> MEAYLNKIDKIEPSDQKIKEEYNKFKYDITKQAIESLRERIPKRIIFFNNLVNVNSEPGSILNVNDLDGVSYKYKINKIEENVRKKHKGNNSSDFDEREKKKDSLDGHVKHFSNNEDSKLIIDDKVLYTHYVPSHKQIYLELEKIK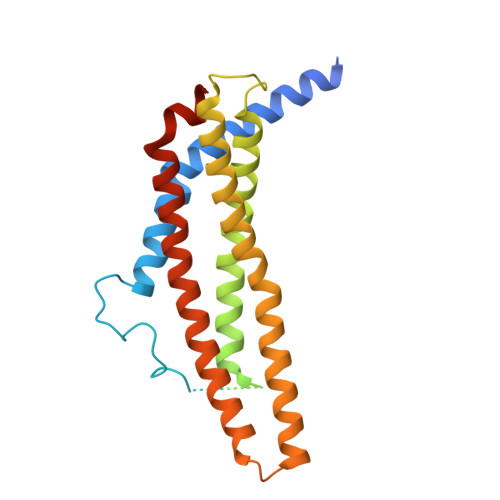TYASELIEIIGNIKLWIQLNVPRIEDGNNFGVGIQEEAIQELARVEESAFNLYDAIVKYYMERAKISTKVLKYPNVSDYQEAVRELDEKEWIHIKITIVDMRNNYIMLYDLLYKNWEKVVKPKNEDAHHRMTF>[2x]ETGTPMMPPVGVQASILSHDTIRITWADNSLPKHQKI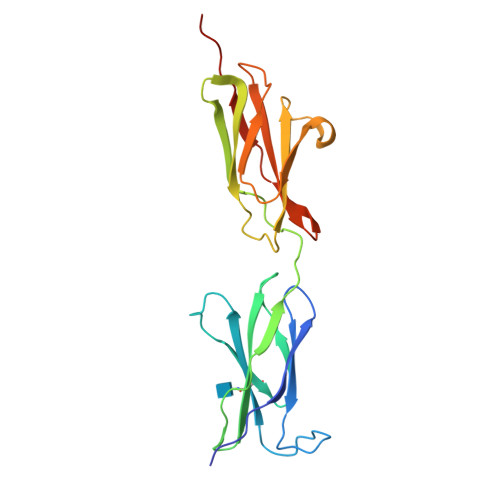TDSRYYTVRWKTNIPANTKYKNANATTLSYLVTGLKPNTLYEFSVMVTKGRRSSTWSMTAHGATFELVPTSPPKDVTVVSKEGKPRTIIVNWQPPSEANGKITGYIIYYSTDVNAEIHDWVIEPVVGNRLTHQIQELTLDTPYYFKIQARNSKGMGPMSEAVQFRTPGTKHHHHHH>[2x]SMDSFKVVLEGPAPWGFRLQGGKDFNVPLSISR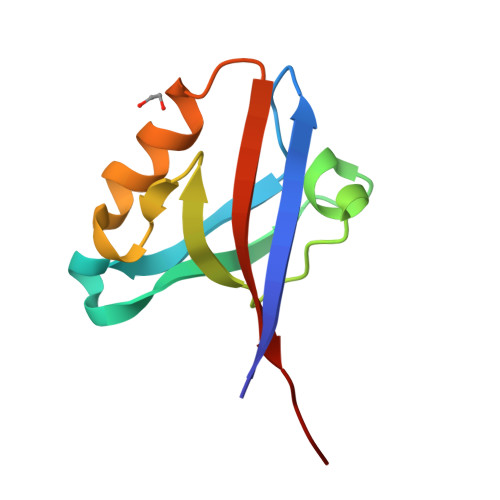LTPGGKAAQAGVAVGDWVLSIDGENAGSLTHIEAQNKIRACGERLSLGLSRAITSL>[8x]MAHHHHHHMSKLAGKVAIVTGASKGIGAAIAKALADEGAAVVVNYASSKAGADAVVSA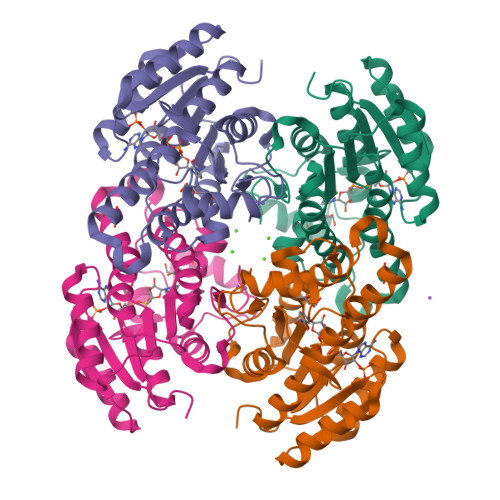ITEAGGRAVAVGGDVSKAADAQRIVDTAIETYGRLDVLVNNSGVYEFAPIEAITEEHYRRQFDTNVFGVLLTTQAAVKHLGEGASIINISSVVTSITPPASAVYSGTKGAVDAITGVLALELGPRKIRVNAINPGMIVTEGTHSAGIIGSDLEAQVLGQTPLGRLGEPNDIASVAVFLASDDARWMTGEHLVVSGGLN(4R)-1-[(3-methylpyridin-4-yl)methyl]-4-(3,4,5-trifluorophenyl)pyrrolidin-2-one 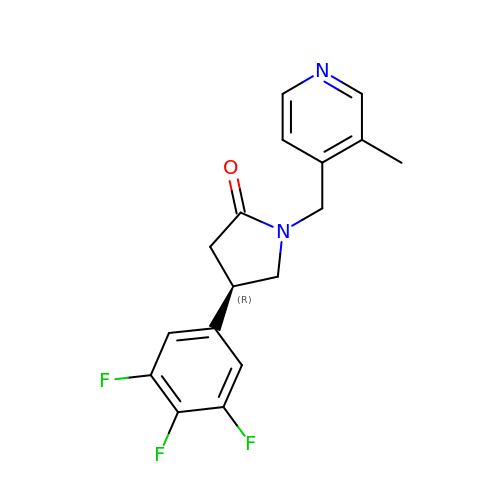| C17 H15 F3 N2 O | RFSDYRVOGWHOFT-ZDUSSCGKSA-N>GHMTPANIAGMVVFIDPGHNGANDASIGRQVPTGRGGTKNCQASGTSTNSGYPEHTFTWETGLRLRAALNALGVRTALSRGNDNALGPCVDERANMANALRPNAIVSLHADGGPASGRGFHVNYSAPPLNAIQAGPSVQFARIMRDQLQASGIPKANYIGQDGLYGRSDLAGLNLAQY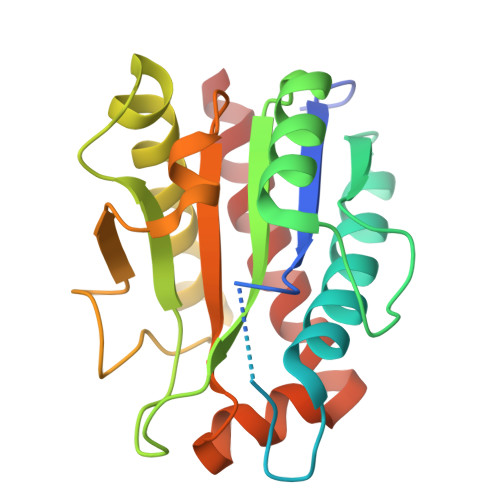PSILVELGNMKNPADSALMESAEGRQKYANALVRGVAGFLATQGQAR[2x]>SNMSAESVAATPESAGGHIRLTSHSGGVGALPIHWGAPTASERGPVVGTTTNRAHRNVIGTHSGSYSIYRALAVASGALSRHHKADLTDTAPTNIIGPYPQWSQPGKIVSLDPWGATVAEVFAAELAAGHDIRPSIAVTKAHVILPEVMEAIQKGRLHPDGRFLLPSGAALVTKAAIEPVWHLPGVAERFHCSETDLRRVLFEETGGMYPELVTRSDLEVFLPPIGGQTVYIFGDARDLADPGVELTARVHDECNGSDVFGSDICTCRPY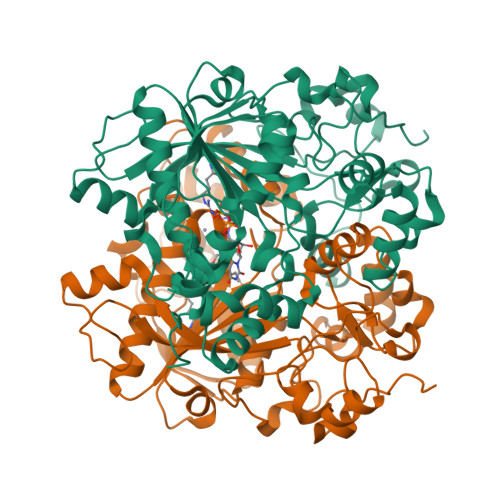LTHAIEECIQGAQRGGVGLVAYSRKEGRALGEVTKFLVYNARKRQVGGDTADQYFARTECVAGVQDMRFQEMMPDVLHWLGVRKIHRLVSMSNMKYDAITGSGIEVVERVDLPADLIPADARVEIDAKMAAGYFTPGAVPDADELAKVKGRELDG[2x]>MIVQLGKASVTWTRADLEAKLAGHARVLIDVGTGDGRFVYRSAGAHPDTYCIGVDPAGERMREVSWRASRKPARGGRPNALFVVASVQALPEELAGLAHTLTLNFPWASLLSALVLPEAPVLEALRRLVRPGGELIALLNQSVFDDRPYAARLGLPELSDAWLDDALRPAYRAAGFEIRTSEIVDGEVPHQTSWGQHLTLA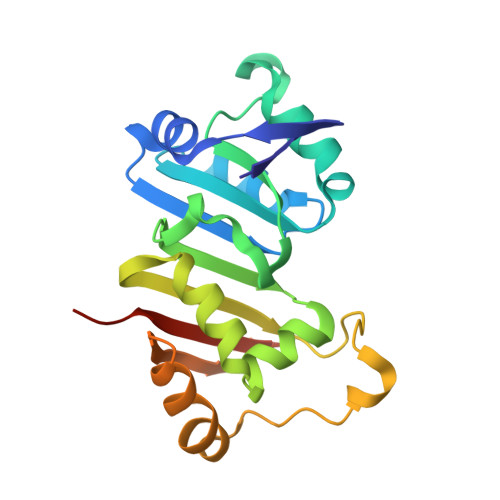SGRRTRLLTAEAIGGSASAAPG[2x]>MNAAAVTPPPEKFNFAEHLLQTNRVRPDKTAFVDDISSLSFAQLEAQTRQLAAALRAIGVKREERVLLLMLDGTDWPVAFLGAIYAGIVPVAVNTLLTADDYAYMLEHSRAQAVLVSGALHPVLKAALTKSDHEVQRVIVSRPAAPLEPGEVDFAEFVGAHAPLEKPAATQADDPAFWLYSSGSTGRPKGVVHTHANPYWTSEL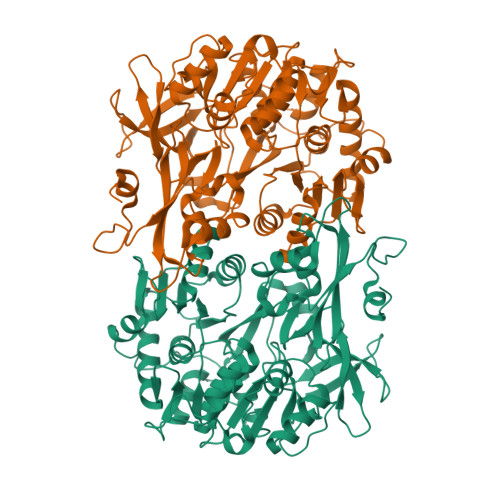YGRNTLHLREDDVCFSAAKLFFAYGLGNALTFPMTVGATTLLMGERPTPDAVFKRWLGGVGGVKPTVFYGAPTGYAGMLAAPNLPSRDQVALRLASSAGEALPAEIGQRFQRHFGLDIVDGIGSTEMLAAFLSNLPDRVRYGTTGWPVPGYQIELRGDGGGPVADGEPGDLYIHGPSSATMYWGNRAKSRDTFQGGWTKSGDKYVRNDDGSYTYAGRTDDMLKVSGIYVSPFEIEATLVQHPGVLEAAVVGVADEHGLTKPKAYVVPRPGQTLSETELKTFIKDRLAPYKYPRSTVFVAELPKTATGKIQRFKLREGVLG[2x]>GSQIHVDTMKVINDPIHGHIELHPLLVRIIDTPQFQRLRYIKQLGGGYYVFPGASHNRFEHSLGVGYLAGCLVHALGEKQPELQISERDVLCVQIAGLCHDLGHGPFSHMFDGRFIPLARPEVKWTHEQGSVMMFEHLINSNGIKPVMEQYGLIPEEDICFIKEQIVGPLESPVEDSLWPYKGRPENKSFLYEIVSNKRNGIDVDKWDYFARDCHHLGIQNNFDYKRFIKFARVCEVDNELRICARDKEVGNLYDMFHTRNSLHRRAYQHKVGNIIDTMITDAFLKADDYIEITGAGGKKYRISTAIDDMEAYTKLTDNIFLEILYSTDPK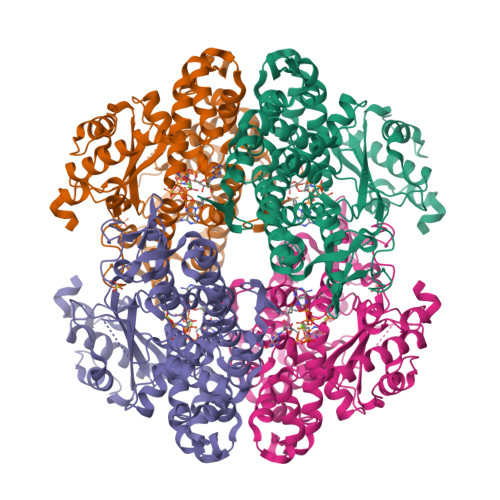LKDAREILKQIEYRNLFKYVGETQPTGQIKIKREDYESLPKEVASAKPKVLLDVKLKAEDFIVDVINMDYGMQEKNPIDHVSFYCKTAPNRAIRITKNQVSQLLPEKFAEQLIRVYCKKVDRKSLYAARQYFVQWCADRNFTKPQDGDVIAPLITPQKKEWNDSTSVQNPTRLREASKSRVQLFKDDPM[16x]>RSYEQMETDGERQNATEIRASVGKMIDGIGRFYIQMCTELKLSDYEGRLIQNSLTIERMVLSAFDERRNKYLEEHPSAGKDPKKTGGPIYRRVDGKWRRELILYDKEEIRRIWRQANNGDDATAGLTHMMIWHSNLNDATYQRTRALVRTGMDPRMCSLMQGSTLPRRSGAAGAAVKGVGTMVMELIRMIKRGINDRNFWRGENGRRTRIAYERMCNILKGKFQTAAQRTMVDQVRESRNPGNAEFEDLIFLARSALILRGSVAHKSCLPACVYGSAVASGYDFEREGYSLVGIDPFRLLQNSQVYSLIRPNENPAHKSQLVWMACHSAAFEDLRVSSFIRGTKVVPRGKLSTRGVQIASNENMETMESST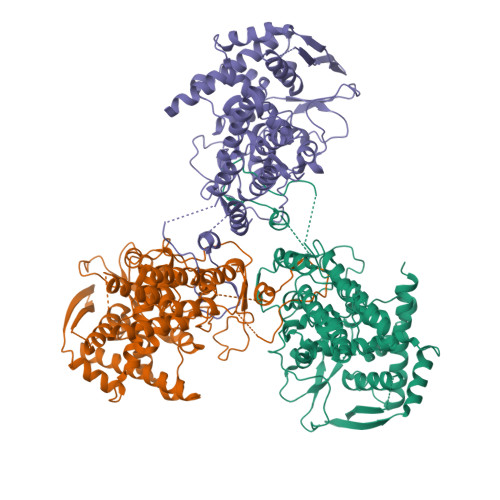LELRSRYWAIRTRSGGNTNQQRASSGQISIQPTFSVQRNLPFDRPTIMAAFTGNTEGRTSDMRTEIIRLMESARPEDVSFQGRGVFELSDEKATSPIVPSFDMSNEGSYFFGDNAEEYDNLEHHHHHH[3x]>MSEFRIHHDVNELLSLLRVHGGDGAEVYIDLLQKNRTPYVTTTVSAHSAKVKIAEFSRTPEDFLKKYDELKSKNTRNLDPLVYLLSKLMEDRETLQYLQQNAKERAELAASAAASSTASFGASATASKISMQELEELRKQLGSVATGPTWQQSLELTRKMLRDKQSKKNSGQRLPVLPAWVYERPALLGDFLPGTGGSADTAVPIGSLPLASQEAAVVEDLLYVLVGVDGRYISAQPLTGRQGRTFLVDPNLDLSIRELVSRILPVAASYSTVTRFIEEKSSFEYGQVNHALAAAMRTLVKEYLVLVTQLEQLQRQGLLSLQKLWFYIQPAMRSLDILASLATSVDKGECIGGATLSLLHDRSFSYTGDSQAQELCLHLTKAASTPYFEILEKWIYRGIIDDPYSEFMVEEHELRKEKIQEDYNDKYWDQRYTVVQRQIPSFLQKMAGKVLSTGKYLNVVRECGHDVTCPVAKEVVYTLKERAYVEQIEKAFSYASKVLLDFLMGEKELLAHLRSIKRYFLMDQGDFFVHFMDLTEEELKKPVDDITPTRLEALLELALRMSTANTDPFKDDLKIDLMPHDLITQLLRVLAIETQQEKAMVHADPTELTLSGLEAFSFDYVVTWPLSLIINRKALTRYQMLFRHMFYCKHVERQLCSVWISNKAAKRFSLHSAKWFAGAFTLRQRMLNFVQNIQSYMMFEVMEPTWHVLEQNLRSASNIDDVLGHHASFLDNCLKDCMLTNPELLRVFSKLMSVCVMFTNCLQRFTQSMKLDSELGHPALEPGAMLGPPTEAERAEERARKELARKCLAEHVDAPQLASSFEATITKFDKNFSAHLLDLLARLSIYSTSDCEHGMASVISRLDFNGFYTERLERLSAERSQKAAPPVPGPRGPPALVPRVAVTAQ[5x];>[5x]MATPDQKSPNVLLQNLCCRILGKSEADVAQQFQYAVRVIGSNFAPTVERDEFLVAEKIKKELTRQRREADAALFSELHRKLHSQGVLKNKWSILYLLLSLSEDPRKQPSKVSGYAALFAQALPRDAHSTPYYYARPQSLPLNYQERGAPSAQSAGSAGSSGVSSLGTYALNGPTPPPPPPALLPGQPLPAPGVGDGLRQQLGSRLAWTLTASQPSLPSTTSKAVPSSGSRGAARPRREGDAAAGAVEVTEAALVRDILYVFQGIDGKHVKMSNADNCYTVEGKANLSKSLRDTAVRLAELGWLHNKIRKYTDQRSLDRSFGLVGQSFCAALHQELREYYRLLSVLHSQLQLEDDQGVNLGLESSLTLRRLLVWTYDPKMRLKTLAALVDHCQGRKGGELASAVHAYTKTGDPYARSLVQHILSLVSHPVLSFLYRWIYDGELEDTYHEFFVASDPAVKADRLWHDKYALRKPMIPSFMTMDQCRKVLLIGKSINFLHQVCHDQTPTTKMIAVTKSAESPQDAADLFTDLENAFQGKIDAAYFETSKYLLDVLNKKYSLLDHMQAMRRYLLLGQGDFIRHLMDLLKPELVRPATTLYQHNLTGILETAVRATNAQFDSPEILKRLDVRLLEVSPGDTGWDVFSLDYHVDGPIATVFTRECMSHYLRAFNFLWRAKRVEYILTDIRKGHMCNARLLRSMPEFSGVLHHCHILASEMVHFIHQMQYYVTFEVLECSWDELWNRVQRAQDLDHIIAAHEAFLGTVISRCLLDSDSRALLNQLRAVFDQIIELQNTQDAIYRAALEELQRRLQFEEKKKQREAEGQWGVSAAEEEQEKRRVQEFQESIPKMCSQLRILTHFYQGVVQQFLVSLTTSSDESLRFLSFRLDFNEHYRAREPRLRVSLGTRGRRSSHT;>MIHELLLALSGYPGSIFTWNKRGGLQVSQDFPFLHPSETSVLNRLCRLGTDYIRFTEFIEQYTGHVQQQDHHPSQQGQGGLHGIYLRAFCTGLDSVLQPYRQALLDLEQEFLADPHLSISHINYSLDQFQLLFPSVMVVVEQIKSQKIHGCQILETVYKHSCGGLPPVRSALEKILAVCHGVMYKQLSAWMLHGLLLDQHEEFFIKQGPSSGNVSAQPEEDEEDLGIGGLTGKQLRELQDLRLIEEENMLAPSLKQFSLRVEILPSYIPVRVAEKILFVGESVQMFENQNVNLTRKGSILKDQEDTFAAELHRLKQQPLFSLVDFEQVVDRIRSTVAEHLWKLMVEESDLLGQLKIIKDFYLLGRGELFQAFIDTAQHMLKTPPTAVTEHDVNVAFQQSAHKVLLDDDNLLPLLHLTIEYHGKEHKADATQAREGPSRETSPREAPASGWAALGLSYKVQWPLHILFTPAVLEKYNVVFKYLLSVRRVQAELQHCWALQMQRKHLKSNQTDAVKWRLRNHMAFLVDNLQYYLQVDVLESQFSQLLHQINSTRDFESIRLAHDHFLSNLLAQSFILLKPVFHCLNEILDLCHSFCSLVSQNLGPLDERGAAQLSILVKGFSRQSSLLFKILSSVRNHQINSDLAQLLLRLDYNKYYTQAGGTLGSFGM[2x];> MASPAPSWTRLDPQQERDVRELIRLVSGVQDEADPNFQLALHFAWSNFRFHRFLDVNSHKVEKTIEGIYEKFIIHSDLSKAASWKRLTDEFLNASLPSIKEIKTDAHYSILSLLLCLSDSPSNSNYVETPRNKEVEKKDDFDWGKYLMEGEEIDLGPNVDTPNWSEESEDEDDPQPLSREDSGIQVDRTPLEEQDQSRKPASRVSWKVDEPDARSWLEQHVVRQYWTTRSSKFPHSLHLHSNLAAVWDQHLYSSDPLYVPDDRVSVTETQVIRETLWLLSGVKKLFIFQLIDGKVAVRNNIMVTHLTHSCLRSVLEQIAAYGQVVFRLQEFIDEVMGHSSESTLPGNGSVPKKSTDAPFRTYQAFMWALYKYFISFKEELSEIEKCIINNDTTVTLAIVVDKLSPRLAQLKVLHKVFSTGVAEVPPDTRNVVRASHLLNTLYKAILEYDNVGEASEQTVSLLFSLWVETVRPYLQIVDEWIVHGHLCDGAREFIIQRNKNVPVNHRDFWYATYTLYSVSEKTENEEKMSDNASASSGSDQGPSSRQHTMVSFLKPVLKQIIMAGKSMQLLKNLQCAESTTCQAMARDAERKSLYTLFLESVQSRLRHGEDATAQALTEQQATRETLIKMQSIAERHLELDDVHDPLLAINFARLYLEQSDFHEKFAGGDICVDRSSESVTCQTFELTLRSCLYPHIDKQYLDCCGNLMRTLKKDYRLVEYLQAMRNFFLMEGGDTMYDFYTSIFDKIREKETWQNVSFLNVQLQEAVGQRYPEDSSRLSISFENTDTAKKKLPVHTLDGLTLSYKVPWPVDIVISLECQKIYNQVFLLLLQIKWAKYSLDVLLFGELASSAEKPQSKEGLLSGQDTAAQFGPQKEPVRQQIHRMFLLRVKLMHFVNSLHNYIMTRILHSTGLEFQHQVEEAKDLDQLIKIHYRYLSTIHDRCLLREKVSFVKEAIMKVLNLALMFADGWQAGLGAWHGISSAVTHGWHGTKLNIFSAVNTSDLIVIHFHHMQLRNRNLFWTVLKPLVYYLDKWILFPLGIIG;> MASVPQLLDDLCEALLPAAKAHLGQRRGSRKRAKQSLKKVAYNALFTNLFQDEARKLQPDLPRLPVKNRILMLSFDLRVGGLAAEADRLEELVEGLETAPRGPLAELGSVLDLLVQLAGSGPPRVLQRRRDYFLPKEHVGRNVRYGGYDCCHLSGIEADVRSIISGEEELCRDLIRKTLQVMEAAPGTGLPAFGLSSYGDPYGDRFERDTRVSLFGALVHSRTADLDVRLDLPPVPDSADVSGLAIKVPLSVDQSEDEGFQSAPNLTPDSQSEPGVTPDIDLWEAVLTYEASRRRCWEQIGCPPGHREEPYLTEAGRDAFDRFCRLRQGELQVLGGALLQAPQPVLVKESELVKDTLNVLLGVVSATFSLCQPAQAFTVKRGVHVSGASPESVSSLLSEVAECGTHYARLSDFSLQPVLDSSCSKGLVFQAFTSGLRRYLQYYRACVLSTPPTLSLLTIGFLFKKLGRQLRYLAELCGVGTALPGTGGGEPRAAFPTGVRLLSYLYQEALDNCSNEHYPVLLSLLKTSCEPYTRFIHDWVYSGVFRDVYGEFMIQVNHEYLGCRDKSYWTHGYVLVSKEVEACVPVFLKHVAHDVYVCGKTINLLKLCCPRHYLCCSDVPVPRISVIFSLEELKDIEKDCAIYVGRMERVARHSSLSKEEKELRMEIAKQELIVHAREAASRVLSALSDRQMSERMALDARKREQFQRLKEQFMRDQERRRAARQEELDDDFSYARELRDRERRLKALEEQLERKARQALVDHYSKLSAEAARRERKALWRVQRHRLADARRRFLLEEEKRVQVMPSCSWERNQGALVFQASLPCPEHPDGGGGCGSGPSEQPKAARDGPRGPSRLMPQLPESPAEAACGLLSVGLSIRDFLPTAQGAEQPLHTGSALVLEEALQTIGSDLPPPAPSAAVGTGPSGPQEYDFRTILRPAVATSAFPGPLQSTGGGLGSEGQPQWEDTHVQLDMCVLDGQVALPHACSPQKTSPQEGSQAMGQLLRQVSEGDVPTGGYASGTAPSRPRWNVHGHVSDASIKVGENVCDVVPSRPRWNVHGHVSDASIKVGENVCDVVPSRPRWNVHGHVSDASIKVGENVCDVVPSRPRWNIHGHVSDASIKVGENVCDVVPSRPRWNVHGHVSQSQVTLGVLSGEAEPIVPWPHQTPPDHGSQSGLSLGAQSPAQEGEPQPAAETAVEGAESGPQASPTAGAGSSLLSGSRLGPEARPPPPPPHLFCPGRSEDTVDLPASCRPSSQVRGQGLGVGGESSAGCPSHPACPFMGNEGSVPGPGVDTQSSPGLGEEAAQRWGMEQAYLAGLAGQYRLEQYPDSYEAMSEPPVARLLHHGLPRAFALPEDSGVQPDTDETAVQLSELLPLPVLMKHSVTAPLAAHVSLVNKAAVDYFFVELHLGAHFEALRHFLLMEDGEFAQSLSDLLFEKLGAGQTPGELLSPLVLNSVLSKALQYSLHGDTPHAANLSFALKFLPEAFAPNAPDVLSCLELRYKVDWPLNIVVTEGCLSRYSGIFSFLLQLKLMMWTLKDVCFHLKRTARMSHVASSVQFRQLQLFKHEMQHFVKVIQGYIANQILHVTWCEFRARLASVGDLEEIQRAHAEYLHKAVFRGLLTEKAAPAMNIIHSLFSLVLKFRSQLISQPWGLAGGPHGAEHPNFALMQQSYSTFKYYSHFLFKVVSKLVNRGYQPHLEDFLLRINFNNYYQDA;>MAGNSGSGAAAAANLNAVRETMDVLLEISRILNTGLDMETLSICVRLCEQGINPEALSSVIKELRKATEALKAAENMTS[3x];> MAAPGAGPGPGAPPGLEAALQKLALRRKKVLSAEETELFELAQAAGGAMDPEVFKILVDLLKLNVAPLAVFQMLKSMCAGQRLASEPQDPVAVPLPTTSVPETRGRNRGSSALGGGPALAERSGREGSSQRMPRQPSATRLPKGGGPGKSPTRST;>[14x]MPREIITLQLGQCGNQIGFEFWKQLCAEHGISPEGIVEEFATEGTDRKDVFFYQADDEHYIPRAVLLDLEPRVIHSILNSPYAKLYNPENIYLSEHGGGAGNNWASGFSQGEKIHEDIFDIIDREADGSDSLEGFVLCHSIAGGTGSGLGSYLLERLNDRYPKKLVQTYSVFPNQDEMSDVVVQPYNSLLTLKRLTQNADCVVVLDNTALNRIATDRLHIQNPSFSQINQLVSTIMSASTTTLRYPGYMNNDLIGLIASLIPTPRLHFLMTGYTPLTTDQSVASVRKTTVLDVMRRLLQPKNVMVSTGRDRQTNHCYIAILNIIQGEVDPTQVHKSLQRIRERKLANFIPWGPASIQVALSRKSPYLPSAHRVSGLMMANHTSISSLFESSCQQYDKLRKREAFLEQFRKEDIFKENFDELDRSREVVQELIDEYHAATRPDYISWGTQEQ;>[2x]MMDLVLEEDVTVPGTLSGCSGLVPSVPDDLDGINPNAGLGNGLLPNVSEETVSPTRARNMKDFENQITELKKENFNLKLRIYFLEERMQQEFHGPTEHIYKTNIELKVEVESLKRELQEREQLLIKASKAVESLAEAGGSEIQRVKEDARKKVQQVEDLLTKRILLLEKDVTAAQAELEKAFAGTETEKALRLRLESKLSEMKKMHEGDLAMALVLDEKDRLIEELKLSLKSKEALIQCLKEEKSQMACPDENVSSGELRGLCAAPREEKERETEAAQMEHQKERNSFEERIQALEEDLREKEREIATEKKNSLKRDKAIQGLTMALKSKEKKVEELNSEIEKLSAAFAKAREALQKAQTQEFQGSEDYETALSGKEALSAALRSQNLTKSTENHRLRRSIKKITQELSDLQQERERLEKDLEEAHREKSKGDCTIRDLRNEVEKLRNEVNEREKAMENRYKSLLSESNKKLHNQEQVIKHLTESTNQKDVLLQKFNEKDLEVIQQNCYLMAAEDLELRSEGLITEKCSSQQPPGSKTIFSKEKKQSSDYEELIQVLKKEQDIYTHLVKSLQESDSINNLQAELNKIFALRKQLEQDVLSYQNLRKTLEEQISEIRRREESFSLYSDQTSYLSICLEENNRFQVEHFSQEELKKKVSDLIQLVKELYTDNQHLKKTIFDLSCMGFQGNGFPDRLASTEQTEEAKKSRLPILIKPSRSLGNMYRLPATQEVVT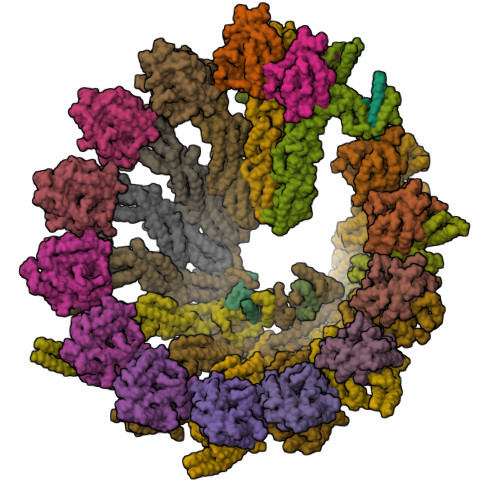QLQSQILELQGELKEFKTCNKQLHQKLILAEAVMEGRPTPDKTLLNAQPPVGAAYQDSPGEQKGIKTTSSVWRDKEMDSDQQRSYEIDSEICPPDDLASLPSCKENPEDVLSPTSVATYLSSKSQPSAKVSVMGTDQSESINTSNETEYLKQKIHDLETELEGYQNFIFQLQKHSQCSEAIITVLCGTEGAQDGLSKPKNGSDGEEMTFSSLHQVRYVKHVKILGPLAPEMIDSRVLENLKQQLEEQEYKLQKEQNLNMQLFSEIHNLQNKFRDLSPPRYDSLVQSQARELSLQRQQIKDGHGICVISRQHMNTMIKAFEELLQASDVDYCVAEGFQEQLNQCAELLEKLEKLFLNGKSVGVEMNTQNELMERIEEDNLTYQHLLPESPEPSASHALSDYETSEKSFFSRDQKQDNETEKTSVMVNSFSQDLLMEHIQEIRTLRKRLEESIKTNEKLRKQLERQGSEFVQGSTSIFASGSELHSSLTSEIHFLRKQNQALNAMLIKGSRDKQKENDKLRESLSRKTVSLEHLQREYASVKEENERLQKEGSEKERHNQQLIQEVRCSGQELSRVQEEVKLRQQLLSQNDKLLQSLRVELKAYEKLDEEHRRLREASGEGWKGQDPFRDLHSLLMEIQALRLQLERSIETSSTLQSRLKEQLARGAEKAQEGALTLAVQAVSIPEVPLQPDKHDGDKYPMESDNSFDLFDSSQAVTPKSVSETPPLSGNDTDSLSCDSGSSATSTPCVSRLVTGHHLWASKNGRHVLGLIEDYEALLKQISQGQRLLAEMDIQTQEAPSSTSQELGTKGPHPAPLSKFVSSVSTAKLTLEEAYRRLKLLWRVSLPEDGQCPLHCEQIGEMKAEVTKLHKKLFEQEKKLQNTMKLLQLSKRQEKVIFDQLVVTHKILRKARGNLELRPGGAHPGTCSPSRPGS We describe a general approach to bind such segments in β-strand and β-hairpin conformations using de novo designed scaffolds that contain deep peptide-binding clefts. To design binders to peptides in extended β-strand conformations, we sought to create scaffolds that could provide β-strand pairing interactions to all the backbone amide and carbonyl atoms of the peptide, such that the peptide strand complements a β-sheet on the scaffold. Starting from FoldIt designed proteins with mixed α/β topology, we designed additional strands and helices to create scaffolds with a single central β-strand missing from an extended β-sheet. The sheet is buttressed by α-helices that pack on one another to support the structure in the absence of the bound peptide.

We obtained a 2.3-Å-resolution crystal structure of a variant of C104, C104.1, where all the surface residues outside the interface were redesigned using ProteinMPNN36. The crystal structure recapitulates the designed model, with both individual domains clamping the peptide in a β-strand conformation. The individual domains superimpose well with the design model. The majority of the peptide is resolved in the electron density and binds in a β-strand conformation with the apolar residues buried in the designed cleft. A deviation from the designed model at helix 3 shifts Tyr91 towards the peptide binding pocket in the crystal structure partially occluding it. As a result, peptide residue Ile8 is displaced and the last few residues of the peptide are disordered in the crystal and are not modeled. For design C104, we confirmed binding in an orthogonal SEC binding assay. Single-amino acid substitution of the buried residue Val6 in the peptide of C104 to arginine completely disrupted binding in BLI, suggesting that the designed binding mode is recapitulated. While the apo state is dynamic, the X-ray crystal structure of a designed binde−peptide complex is highly ordered and very close to the design model. The shape-complementary binding pockets in our designs nearly completely engulf the bound peptide.

> GQRIRVRI;> GSVTFEFENLSEEAAEKVKKYVKEVAEKLGVEVKVEEEEGKLKIYVENLKEEDALDIFKYAALAAELDQEYLDMVEAAIKAYHLFKEYDENATIEITIDDEGIEVKVESGDRVVTLKFKNVSKEEVEEAVKEALKQLEAGQKKVEVEVEGGS>KAGPTLEELLGQCTAENRHHEYLCDSQGKEML[2x];>[4x]MTTYCPARGDVILLDFNPQSGHEQAGKRPALVVSDDLFNQVTGFAVVCPITNQIKGYPFEVPVDGTTKTTGVILADQVKSLDWKARAA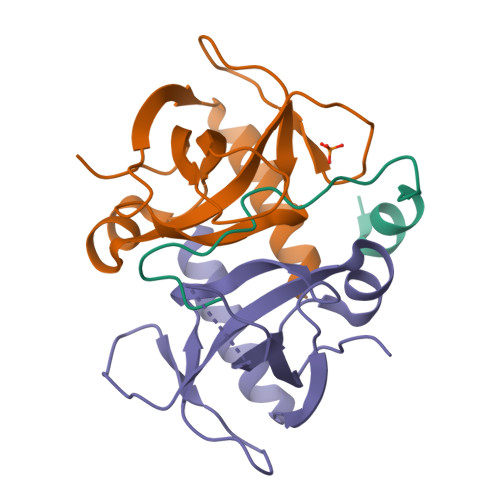RTVDSVSGETVTTVVDMVSKIIKA N-{(2R)-4-(methylamino)-4-oxo-2-[4-(phosphonooxy)benzyl]butanoyl}-L-valyl-L-aspartamide 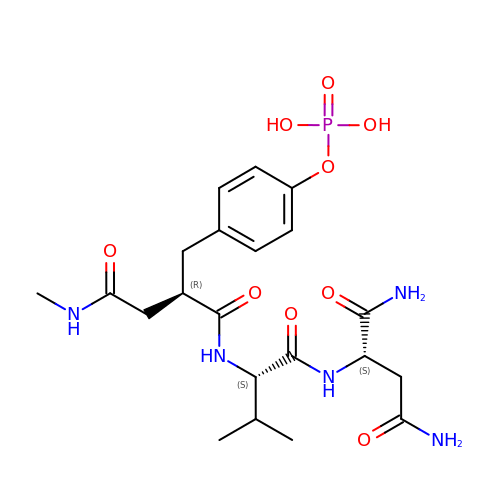| C21 H32 N5 O9 P | CCEFGGFBPGVHRR-XUWXXGDYSA-N>MANEVIKCKAAVAWEAGKPLSIEEIEVAPPKAHEVRIKIIATAVCHTDAYTLSGADPEGCFPVILGHEGAGIVESVGEGVTKLKAGDTVIPLYIPQCGECKFCLNPKTNLCQKIRVTQGKGLMPDGTSRFTCKGKTILHYMGTSTFSEYTVVADISVAKIDPLAPLDKVCLLGCGISTGYGAAVNTAKLEPGSVCAVFGLGGVGLAVIMGCKVAGASRIIGVDINKD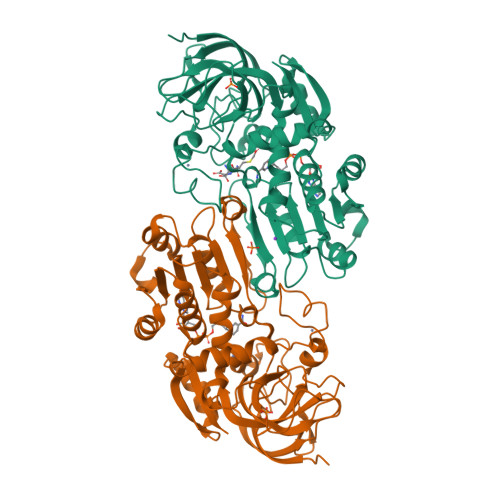KFARAKEFGATECINPQDFSKPIQEVLIEMTDGGVDYSFECIGNVKVMRAALEACHKGWGVSVVVGVAASGEEIATRPFQLVTGRTWKGTAFGGWKSVESVPKLVSEYMSKKIKVDEFVTHNLSFDEINKAFELMHSGKSIRTVVKI[2x]> IVGGYTCAANSIPYQVSLNSGSHFCGGSLINSQWVVSAAHCYKSRIQVRLGEHNIDVLEGNEQFINAAKIITHPNFNGNTLDNDIMLIKLSSPATLDSRVATVSLPRSCAAAGTECLISGWGNTKSSGSSYPSLLQCLKAPVLSDSSCKSSYPGQITGNMICVGFLEGGKDSCQGDSGGPVVCNGQLQGIVSWGYGCAQKNKPGVYTKVCNYVNWIQQTIAAN;> FDVNSHTTPCGPVTCSGAQMCEVDKCVCSDLHCKVKCEHGFKKD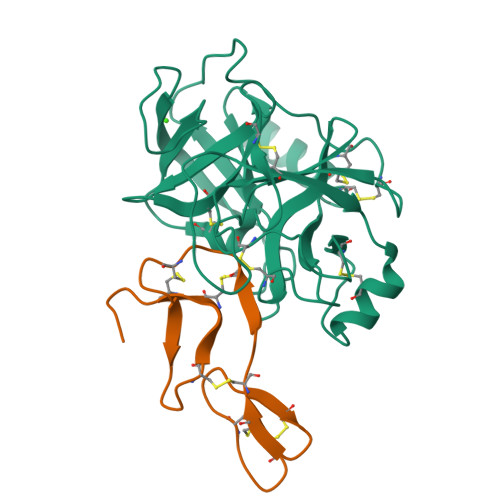DNGCEYACICADAPQ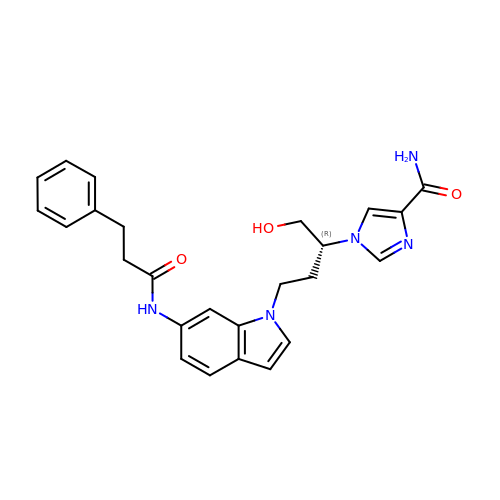1-((1R)-1-(HYDROXYMETHYL)-3-{6-[(3-PHENYLPROPANOYL)AMINO]-1H-INDOL-1-YL}PROPYL)-1H-IMIDAZOLE-4-CARBOXAMIDE | C25 H27 N5 O3 | GUYYFMCFEPDDFL-OAQYLSRUSA-N5'-O-[(S)-butoxy(hydroxy)phosphoryl]adenosine | C14 H22 N5 O7 P | 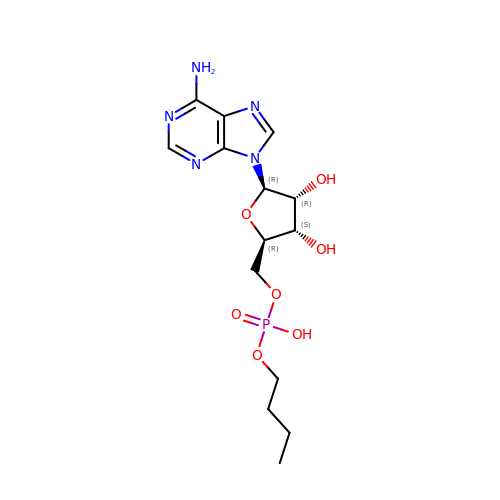VOMQEXIAZJZJAB-IDTAVKCVSA-N>GHMVTMSTEPVSASDKYQKISQLEHILKRPDTYIGSVETQEQLQWIYDEETDCMIEKNVTIVPGLFKIFDEILVNAADNKVRDPSMKRIDVNIHAEEHTIEVKNDGKGIPIEIHNKENIYIPEMIFGHLLTSSNYDDDEKKVTGGRNGYGAKLCNIFSTEFILETADLNVGQKYVQKWENNMSICHPPKITSYKKGPSYTKVTFKPDLTRFGMKELDNDILGVMRRRVYDINGSVRDINVYLNGKSLKIRNFKNYVELYLKSLEKKRQLDNGEDGAAKSDIPTILYERINNRWEVAFAVSDISFQQISFVNSIATTMGGTHVNYITDQIVKKISEILKKKKKKSVKSFQIKNNMFIFINCLIENPAFTSQTKEQLTTRVKDFGSRCEIPLEYINKIMKTDL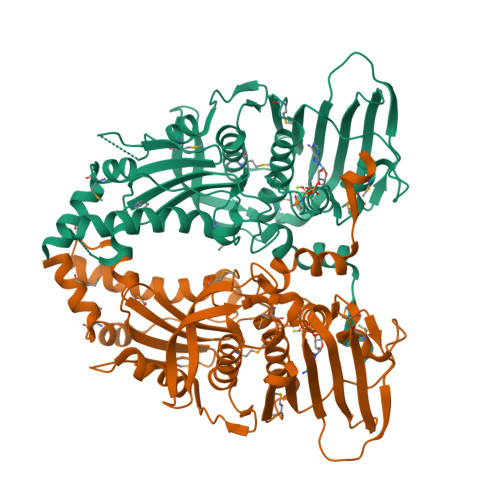ATRMFEIADANEENALK[2x]>[4x]PSETPQAEVGPTGCPHR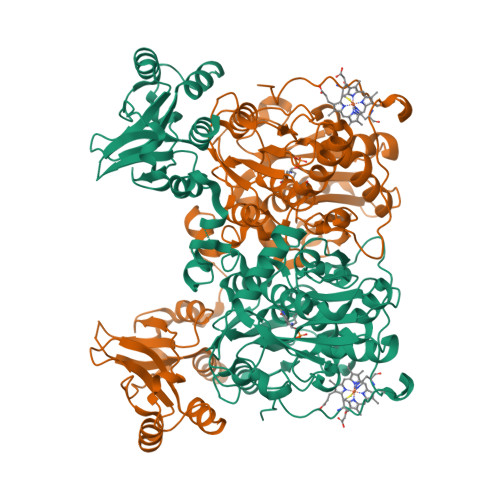SGPHSAKGSLEKGSPEDKEAKEPLWIRPDAPSRCTWQLGRPASESPHHHTAPAKSPKILPDILKKIGDTPMVRINKIGKKFGLKCELLAKCEFFNAGGSVKDRISLRMIEDAERDGTLKPGDTIIEPTSGNTGIGLALAAAVRGYRCIIVMPEKMSSEKVDVLRALGAEIVRTPTNARFDSPESHVGVAWRLKNEIPNSHILDQYRNASNPLAHYDTTADEILQQCDGKLDMLVASVGTGGTITGIARKLKEKCPGCRIIGVDPEGSILAEPEELNQTEQTTYEVEGIGYDFIPTVLDRTVVDKWFKSNDEEAFTFARMLIAQEGLLCGGSAGSTVAVAVKAAQELQEGQRCVVILPDSVRNYMTKFLSDRWMLQKGFLKEEDLTEKKPWWWHLRVQELGLSAPLTVLPTITCGHTIEILREKGFNQAPVVDEAGVILGMVTLGNMLSSLLAGKVQPSDQVGKVIYKQFKQIRLTDTLGRLSHILEMDHFALVVHEQIQYHSTGKSSQRQMVFGVVTAIDLLNFVAAQERDQKLEHHHHHH>[6x]PP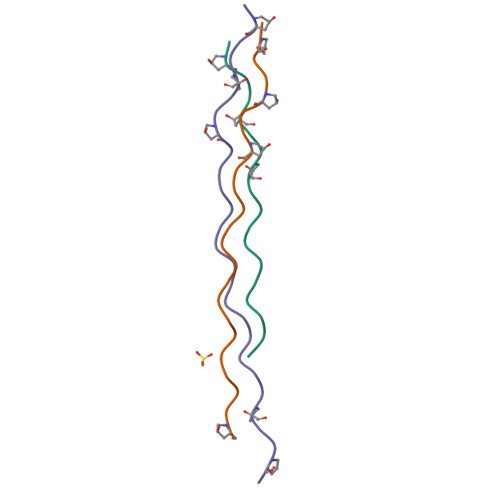GPPGPPGFDGRNGEKGETGPPGPPGPPG> MNDIAHNLAQVRDKISAAATRCGRSPEEITLLAVSKTKPASAIAEAIDAGQRQFGENYVQEGVDKIRHFQELGVTGLEWHFIGPLQSNKSRLVAEHFDWCHTIDRLRIATRLNDQR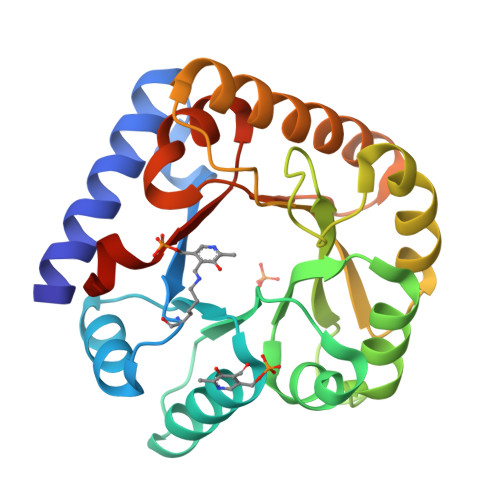PAELPPLNVLIQINISDENSKSGIQLAELDELAAAVAELPRLRLRGLMAIPAPESEYVRQFEVARQMAVAFAGLKTRYPHIDTLSLGMSDDMEAAIAAGSTMVRIGTAIFGARDYSKK> GUGUGCCCGGCAUGGGUGCAGUCUAUAGGGUGAGAGUCCCGAACUGUGAAGGCAGAAGUAACAGUUAGCCUAACGCAAGGGUGUCCGUGGCGACAUGGAAUCUGAAGGAAGCGGACGGCAAACCUUCGGUCUGAGGAACACGAACUUCAUAUGAGGCUAGGUAUCAAUGGAUGAGUUU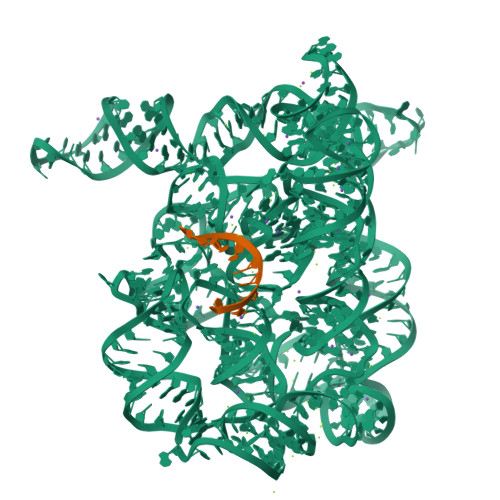GCAUAACAAAACAAAGUCCUUUCUGCCAAAGUUGGUACAGAGUAAAUGAAGCAGAUUGAUGAAGGGAAAGACUGCAUUCUUACCCGGGGAGGUCUGGAAACAGAAGUCAGCAGAAGUCAUAGUACCCUGUUCGCAGGGGAAGGACGGAACAAGUAUGGCGUUCGCGCCUAAGCUUGAACCGCCGUAUACCGAACGGUACGUACGGUGGUGUGAGAGGAGUUCGCUCUACUCUAU;> UGUUAUUUU Besides NADH-dependent ferredoxin: NADP+ oxidoreductase (Nfn), the best studied FBEB system is the electron transferring flavoprotein/butyryl-CoA dehydrogenase (EtfAB/Bcd) complex, which is a key enzyme in butyrate producing anaerobes. The EtfAB/Bcd complex is composed of subunits EtfA, EtfB and Bcd; each subunit contains one FAD as prosthetic group, termed α-FAD, β-FAD and δ-FAD, respectively. In the applied enzyme machineries, a flavin hydroquinone (HQ or FH−) acts as the bifurcating donor; one electron flows to a high-potential acceptor, whereas the other electron reduces the low potential ferredoxin or flavodoxin. All EtfABs are composed of three domains; domains I and II are components of the A- or α-subunit, and domain III of the B- or β-subunit. α-FAD is located in the mobile domain II and β-FAD sits between the rigid domains I and III.

The EtfAB/Bcd complex was found in a heterododecameric (EtfAB/Bcd)4 state with a molecular mass of ca. 440 kDa. Architecturally, the tetrameric Bcd forms the core of the enzyme complex to which four EtfAB units are peripherally attached. Each EtfAB unit forms two contact areas with a Bcd dimer (the monomers named Bcd1 and Bcd2) that are placed around 50 Å apart from each other. The first contact area is located between the N-terminal domain of Bcd1 and the EtfAB base and is considered as fixed during the reaction cycle. The second contact region is formed between domain II and the Bcd1–Bcd2 dimer. In the determined EtfAB/Bcd structure characterized by a pronounced domain II-Bcd dimer interface, the distance between α-FAD and δ-FAD is 8.4 Å thereby indicating that the EtfAB/Bcd complex is trapped in a dehydrogenase-conducting conformation termed D state. The edge-to-edge distance between the β-FAD and α-FAD isoalloxazines is 37 Å which certainly excludes mutual ET. In the D state, α-FAD is involved in the domain II-Bcd interface and the exposed xylene ring is completely encapsulated by T343, Y346, and Y340 of Bcd2 as well as F155 and E198 of Bcd1. Therefore, domain II is kept in its position by its interactions with Bcd.

>[2x]MGNVLVVIEQRENVIQTVSLELLGKATEIAKDYDTKVSALLLGSKVEGLIDTLAHYGADEVIVVDDEALAVYTTEPYTKAAYEAIKAADPIVVLFGATSIGRDLAPRVSARIHTGLTADCTGLAVAEDTKLLLMTRPAFGGNIMATIVCKDFRPQMSTVRPGVMKKNEPDETKEAVINRFKVEFNDADKLVQVVQVIKEAKKQVKIEDAKILVSAGRGMGGKENLDILYELAEIIGGEVSGSRATIDAGWLDKARQVGQTGKTVRPDLYIACGISGAIQHIAGMEDAEFIVAINKNPEAPIFKYADVGIVGDVHKVLPELISQLSVAKEKG;>MNIVVCIKQVPDTTEVKLDPNTGTLIRDGVPSIINPDDKAGLEEAIKLKEEMGAHVTVITMGPPQADMALKEALAMGADRGILLTDRAFAGADTWATSSALAGALKNIDFDIIIAGRQAIDGDTAQVGPQIAEHLNLPSITYAEEIKTEGEYVLVKRQFEDCCHDLKVKMPCLITTLKDMNTPRYMKVGRIYDAFENDVVETWTVKDIEVDPSNLGLKGSPTSVFKSFTKSVKPAGTIYNEDAKTSAGIIIDKLKEKYII[2x];>[2x]MDLNSKKYQMLKELYVSFAENEVKPLATELDEEERFPYETVEKMAKAGMMGIPYPKEYGGEGGDTVGYIMAVEELSRVCGTTGVILSAHTSLGSWPIYQYGNEEQKQKFLRPLASGEKLGAFGLTEPNAGTDASGQQTTAVLDGDEYILNGSKIFITNAIAGDIYVVMAMTDKSKGNKGISAFIVEKGTPGFSFGVKEKKMGIRGSATSELIFEDCRIPKENLLGKEGQGFKIAMSTLDGGRIGIAAQALGLAQGALDETVKYVKERVQFGRPLSKFQNTQFQLADMEVKVQAARHLVYQAAINKDLGKPYGVEAAMAKLFAAETAMEVTTKAVQLHGGYGYTRDYPVERMMRDAKITEIYEGTSEVQRMVISGKLLK>[2x]MMEQVCDVFDIYAICACCKVESKNEGKKNEVFNNYTFRGLGNKGVLPWKCNSLDMKYFCAVTTYVNESKYEKLKYKRCKYLNKETVDNVNDMPNSKKLQNVVVMGRTSWESIPKKFKPLSNRINVILSRTLKKEDFDEDVYIINKVEDLIVLLGKLNYYKCFIIGGSVVYQEFLEKKLIKKIYFTRINSTYECDVFFPEINENEYQIISVSDVYTSNNTTLDFIIYKKTNNKMLNEQNCIKGEEKNNDMPLKNDDKDTCHMKKLTEFYKNVDKYKINYENDDDDEEEDDFVYFNFNKEKEEKNKNSIHPNDFQIYNSLKYKYHPEYQYLNIIYDIMMNGNKQSDRTGVGVLSKFGYIMKFDLSQYFPLLTTKKLFLRGIIEELLWFIRGETNGNTLLNKNVRIWEANGTREFLDNRKLFHREVNDLGPIYGFQWRHFGAEYTNMYDNYENKGVDQLKNII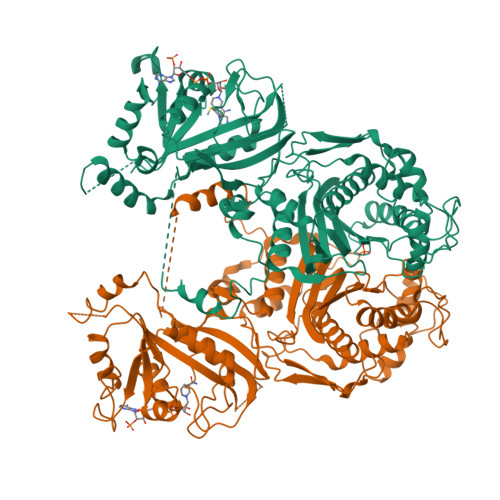NLIKNDPTSRRILLCAWNVKDLDQMALPPCHILCQFYVFDGKLSCIMYQRSCDLGLGVPFNIASYSIFTHMIAQVCNLQPAQFIHVLGNAHVYNNHIDSLKIQLNRIPYPFPTLKLNPDIKNIEDFTISDFTIQNYVHHEKISMDMAA> GSGSGSDIEAYLERIGYKKSRNKLDLETLTDILQHQIRAVPFENLNIHCGDAMDLGLEAIFDQVVRRNRGGWCLQVNHLLYWALTTIGFETTMLGGYVYSTPAKKYSTGMIHLLLQVTIDGRNYIVDAGSGRSYQMWQP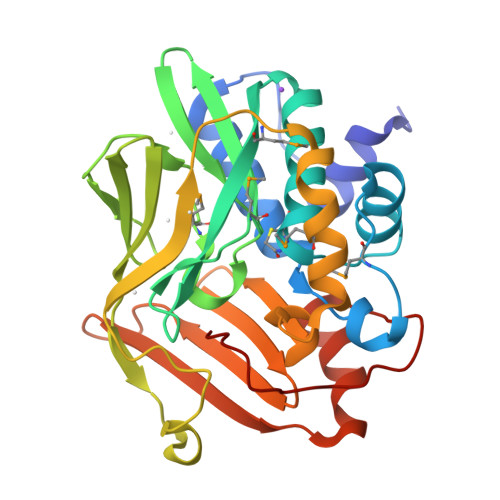LELISGKDQPQVPCVFRLTEENGFWYLDQIRREQYIPNEEFLHSDLLEDSKYRKIYSFTLKPRTIEDFESMNTYLQTSPSSVFTSKSFCSLQTPDGVHCLVGFTLTHRRFNYKDNTDLIEFKTLSEEEIEKVLKNIFNISLQRKLVPKHGDRFFTI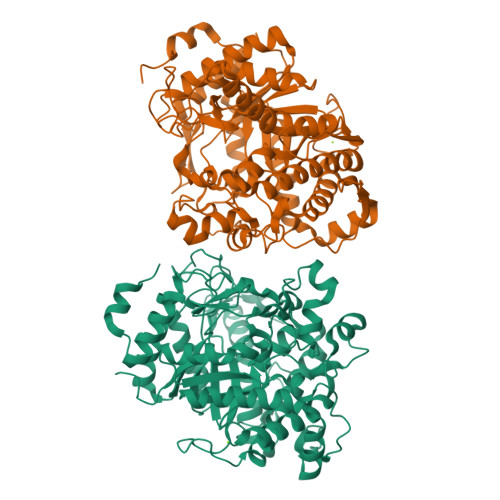>MPFPEKFFWGASSSGFQFEMGDPEGKSIDPNTDWFKWVHDETNIRRGVVSGDLPEHGINYWDLFRSDHELAASIGMNAYRIGIEWSRIFPKPTLDVRVGIELDPEGYITRVEVDDKAIEELDLLANKEAVSRYREIILDLRDRGLKVFVCLNHFTLPLWIHDPIACRDTKLKRGPKGWVDKTTILEFAKYSAYMAWSLGNIVDYWVTFNEPMVVTEAGYFQPEVGFPPGLRNISAFKTACLNIANAHVVAYDLIKKYDKVRADDDSPSAAYVGIVHNIVPIKPYSERKLDLKAADLMNYIHNKWILEFIVRGKIDRSLVGREKYLIDKFKDKLDWLGVNYYTRIVLKGKWVPPLISPVPVIPDIVKGYGFNCTPGGRSLDGMPVSDFGWEVYPQGLSDALDIASEYGKPLIVTENGIADSEDNIRPYFLVSHLKVLEEYVEKKKNVYGYLHWALTDNYEWAQGFKMRFGLTDVDLETKERKPRESSEVFKIIASEKTVPEELVEKYPKPIF[2x]Volume-regulated anion channels (VRACs) are expressed widely in vertebrate cell types where they mediate the efflux of Cl- and organic solutes required for cell volume regulation. 8C-8A(IL125) consists of a 25-amino acid sequence unique to the first intracellular loop, IL1, of LRRC8A inserted into the corresponding region of LRRC8C. Like native VRAC/LRRC8 channels, 8C-8A(IL125) chimeras are activated strongly by cell swelling and low intracellular ionic strength. We demonstrate that the 8C-8A(IL125) chimeric channel is a large-pore seven-subunit heptamer, like homologous pannexin channels.

We obtained five distinct 3D classes for the 8C-8A(IL125) chimera. The most apparent difference between the structures is in the arrangement of the LRRDs. In class 1, all seven LRRDs are arranged circularly with roughly sevenfold symmetry. When the ICD and TMD are viewed from the cytoplasm, 8C-8A(IL125) subunits are organized into two distinct groups, one with four subunits and the other with three subunits. These two groups of subunits associate via a loose interface, while the subunits within each group associate via a tight interface (Figure 3A–D and Figure 3—figure supplements 1–3). In two of the subunits in the class 1 structure, K51 points toward the pore, while D50 points in the opposite direction. In the five other subunits, D50 points toward the pore, and K51 is oriented toward the subunit interface. When K51 points toward the pore, it creates a groove between the subunits. These grooves, located between the subunits forming the loose interface in the class 1 structure, connect the space within the ECD to the membrane-facing surface of the TMD. When D50 points toward the pore, the side chain of K51 occupies this space, closing the groove.

>[7x]MIPVTEFRQFSEQQPAFRVLKPWWDVFTDYLSVAMLMIGVFGCTLQVMQDKIICLPKRVQPAQNHSSLSNVSQAVASTTPLPPPKPSPANPITVEMKGLKTDLDLQQYSFINQMCYERALHWYAKYFPYLVLIHTLVFMLCSNFWFKFPGSSSKIEHFISILGKCFDSPWTTRALSEVSGEDSDPKPAFSKMNGSMDKKSSTVSEDVEGSLVNSQSLKSIPEKFVVDKSTAGALDKKEGEQAKALFEKVKKFRLHVEEGDILYAMYVRQTVLKVIKFLIIIAYNSALVSKVQFTVDCNVDIQDMTGYKNFSCNHTMAHLFSKLSFCYLCFVSIYGLTCLYTLYWLFYRSLREYSFEYVRQETGIDDIPDVKNDFAFMLHMIDQYDPLYSKRFAVFLSEVSENKLKQLNLNNEWTPDKLRQKLQTNAHNRLELPLIMLSGLPDTVFEITELQSLKLEIIKNVMIPATIAQLDNLQELSLHQCSVKIHSAALSFLKENLKVLSVKFDDMRELPPWMYGLRNLEELYLVGSLSHDISRNVTLESLRDLKSLKILSIKSNVSKIPQAVVDVSSHLQKMCIHNDGTKLVMLNNLKKMTNLTELELVHCDLERIPHAVFSLLSLQELDLKENNLKSIEEIVSFQHLRKLTVLKLWHNSITYIPEHIKKLTSLERLSFSHNKIEVLPSHLFLCNKIRYLDLSYNDIRFIPPEIGVLQSLQYFSITCNVESLPDELYFCKKLKTLKIGKNSLSVLSPKIGNLLFLSYLDVKGNHFEILPPELGDCRALKRAGLVVEDALFETLPSDVREQMKTEENLYFQGAAAGDYKDDDDK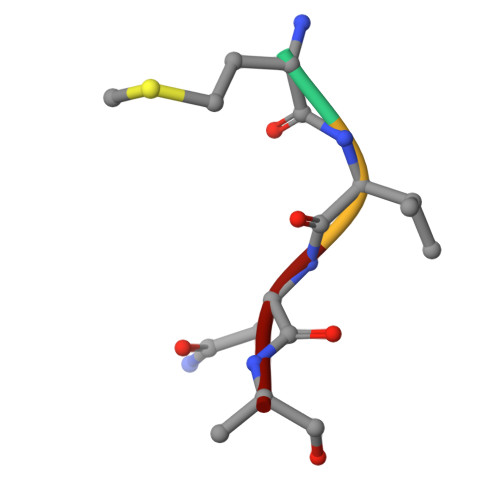> MVNA> MTSVNSAEASTGAGGGGSNPVKSMWSEGATFSANSVTCTFSRQFLIPYDPEHHYKVFSPAASSCHNASGKEAKVCTISPIMGYSTPWRYLDFNALNLFFSPLEFQHLIENYGSIAPDALTVTISEIAVKDVTDKTGGGVQVTDSTTGRLCMLVDHEYKYPYVLGQGQDTLAPELPIWVYFPPQYAYLTVGDVNTQGISGDSKKLASEESAFYVLEHSSFQLL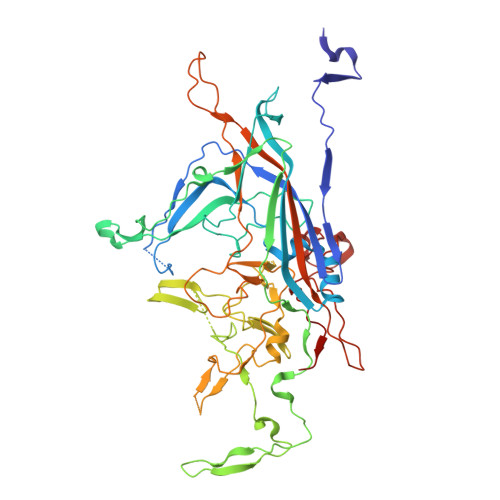GTGGTATMSYKFPPVPPENLEGCSQHFYEMYNPLYGSRLGVPDTLGGDPKFRSLTHEDHAIQPQNFMPGPLVNSVSTKEGDSSNTGAGKALTGLSTGTSQNTRISLRPGPVSQPYHHWDTDKYVTGINAISHGQTTYGNAEDKEYQQGVGRFPNEKEQLKQLQGLNMHTYFPNKGTQQYTDQIERPLMVGSVWNRRALHYESQLWSKIPNLDDSFKTQFAALGGWGLHQPPPQIFLKILPQSGPIGGIKSMGITTLVQYAVGIMTVTMTFKLGPRKATGRWNPQPGVYPPHAAGHLPYVLYDPTATDAKQHHRHGYEKPEELWTAKSRVHPL>GGGTTGCGGAGGGTGGGCC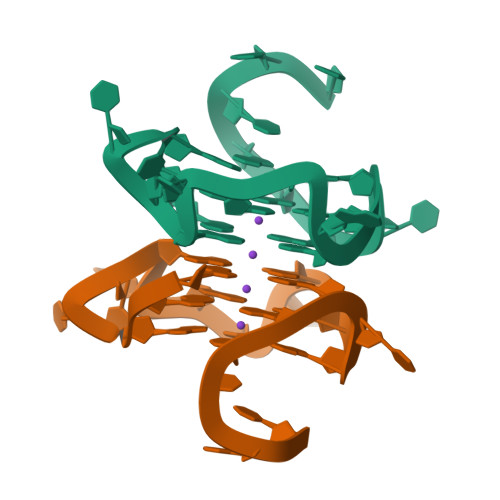T[2x]>HDDHDHDHAHGSLGKHEHGVAQLNVALDGKTLELELDSPAMNLVGFEHAASTDADKAAVAKARAQLEKPLELFALPVTAGCSVASQELRSPLFGDKAPAHAHKEKAGHEHEHEHEHEHGHADIHAHYQLSCEKPELLKLLTLAEFFKRFPATQKIQVQLIGPDGQKGADLAP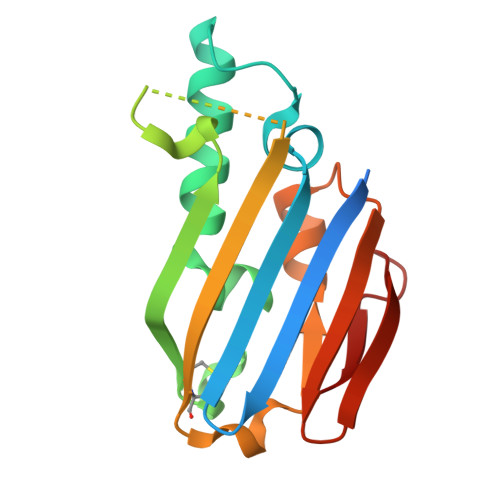ASAELKL[3x]>[2x]MTIQDFQSSGKATVLAVGTAVPPKEFDQSTYPDFYFNVTNCNDKVELKGKFQRICDRSGIKKRHFYLDEEILKANPGMCTYMGASLDVRQNIAVREVPKLAKEAALKAIKEWGQPKSKITHLVFGTTSGVDMPGADFQLL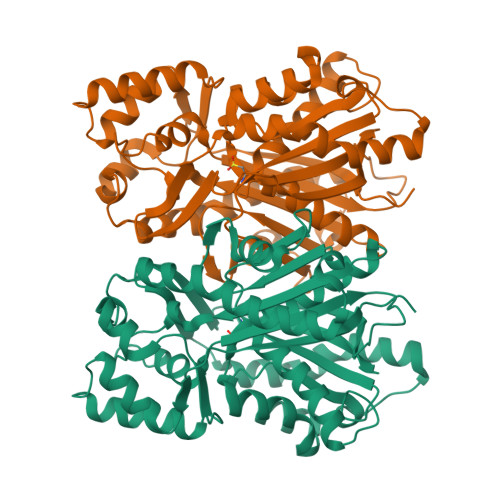KLLGLRPNVKRIMLYQQGCSAGATVTRVAKDLAENNPGARVLVACSEVTAVTFRAPSETHLDGLVGAALFGDGAAALIIGSNPTPVEKPLFEVHWSGQCVLPDSDGAILGHLREAGLVFHLLKDVPGIISKNIEKLLAEPLDYVKSVDEASPAYTDLFWVVHPGGPAILDQVEAKLKLDKDRMQATRDVLAQYGNMSSACVLFVLDQMRKRSVELNKDTTGDGLKWGVMLGFGPGLTVETLLLKSI>[2x]MAEKPKLHYFNARGRMESTRWLLAAAGVEFEEKFIKSAEDLDKLRNDGYLMFQQVPMVEIDGMKLVQTRAILNYIASKYNLYGKDIKERALIDMY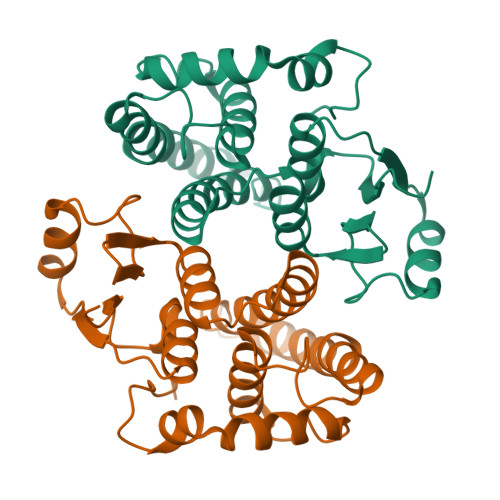IEGIADLGEMILLLPVCPPEEKDAKLALIKEKIKNRYFPAFEKVLHHHGQDYLVGNKLSRADIHLVELLYYVEELDSSLISSFPLLKALKTRISNLPTVKKFLQPGSPRKPPMDEKSLEEARKIFRF> MASWSHPQFEKMGMLEARELLCERDERTLFSGLSFTLNAGEWVQITGSNGAGKTTLLRLLTGLSRPDAGEVLWQGQPLHQVRDSYHQNLLWIGHQPGIKTRLTALENLHF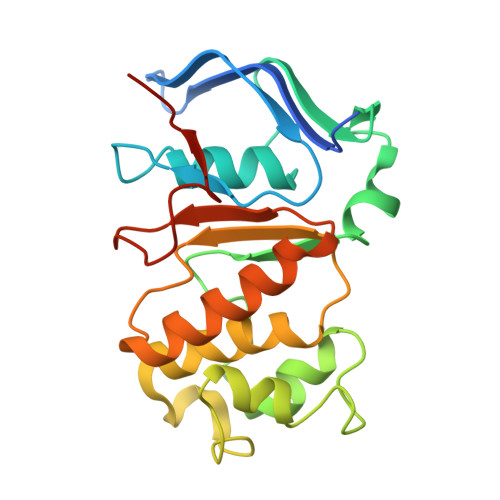YHRDGDTAQCLEALAQAGLAGFEDIPVNQLSAGQQRRVALARLWLTRATLWILDEPFTAIDVNGVDRLTQRMAQHTEQGGIVILTTHQPLNVAESKIRRISLTQTRAA3-deoxy-8-O-phosphono-D-manno-oct-2-ulosonic acid | C8 H15 O11 P | 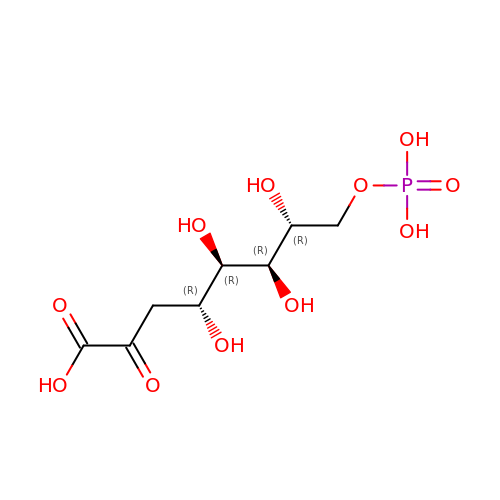RTNBXJBOAIDPME-SHUUEZRQSA-N> GSNNSETPAPGPDSLLALAFPSDPQVSPDGKQVAFVLAQISEEDPAKPDKDFARPRYRSGLWLSEGGAARPLTHAETGRGDSAPRWSPDGQNLAFVRSAGEVKAALMLLPLKGGEARRVTHFKNGVSGPQWSPDGRFIAFTTTADTEDKRDERGEARVLTRPVYRANGADWLPERPAALWLYDVEADKLREWYAPEIGIGALSWWPDSRGVLIVQSEDEWQASQWRQDVYDLPLPTADAPAAPQKLLDWNSAAHGLAPHPDGQRFALIGRPAGKGNTEHAHLYLIENGQHRRLDTGHDHPVGDAVGGDCHVGAFPEGPRWLDGDTLLFSSTVRGSVGLFTAHIGGGVKAYDHDPQGVI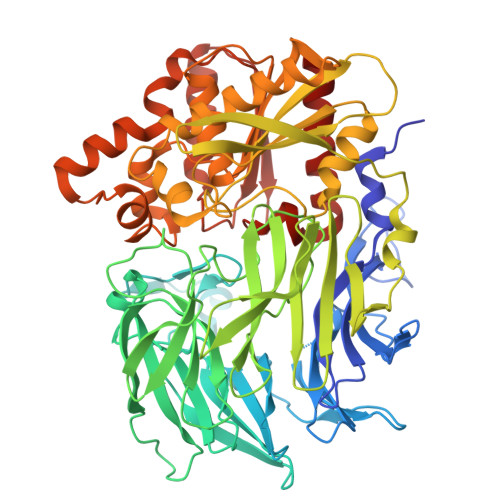SAFTANEHGVALIRESATRFPEVELNGQRVTDLHARFPFPVREPQRVTFETELGEGEGWVLLPEGEQKVPALLNIHGGPHTDYGHGFTHEFQLMAARGYGVCYSNPRGSVGYGQAWVDAIYGRWGTVDADDLLNFFDRCLEAVPRLDAAKTAVMGGAYGGFMTNWITGHTTRFQAAITDRCISNLISFGGTSDIGLRFWDDELGLDFSRRADALKLWDLSPLQYVENVKTPTLIVHSVLDHRCPVEQAEQWYAALHKHQVPVRFVRFPEENHELSRSGRPDRRLTRLNEYFAWLERWL>MGNSGQFLDAAKALQVWPLIEKRTCWHGHAGGGLHTDPKEGLKDVDTRKIIKAMLSYVWPKDRPDLRARVAISLGFLGGAKAMNIVVPFMFKYAVDSLNQMSGNMLNLSDAPNTVATMATAVLIGYGVSRAGAAFFNEVRNAVFGKVAQNSIRRIAKNVFLHLHNLDLGFHLSRQTGALSKAIDRGTRGISFVLSALVFNLLPIMFEVMLVSGVLYYKCGAQFALVTLGTLGTYTAFTVAVTRWRTRFRIEMNKADNDAGNAAIDSLLNYETVKYFNNERYEAQRYDGFLKTYETASLKSTSTLAMLNFGQSAIFSVGLTAIMVLASQGIVAGTLTVGDLVMVNGLLFQLSLPLNFLGTVYRETRQALIDMNTLFTLLKVDTQIKDKVMASPLQITPQTATVAFDNVHFEYIEGQKVLSGISFEVPAGKKVAIVGGSGSGKSTIVRLLFRFYEPQKGSIYLAGQNIQDVSLESLRRAVGVVPQDAVLFHNTIYYNLLYGNISASPEEVYAVAKLAGLHDAILRMPHGYDTQVGERGLKL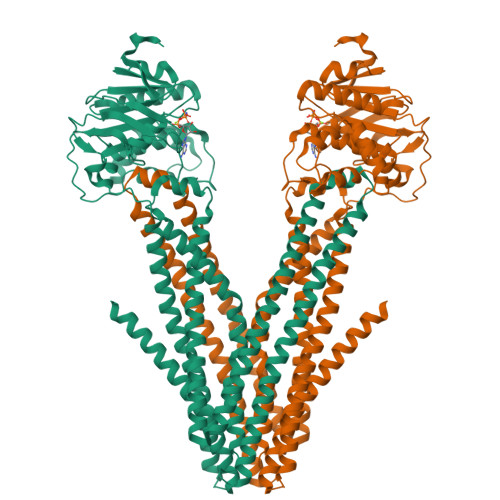SGGEKQRVAIARAILKDPPVILYDEATSSLDSITEETILGAMKDVVKHRTSIFIAHRLSTVVDADEIIVLDQGKVAERGTHHGLLANPHSIYSEMWHTQSSRVQNHDNPKWEAKKENISKEEERKKLQEEIVNSVKGCGNCSDYKDDDDKDYKDDDDK[2x]>[2x]M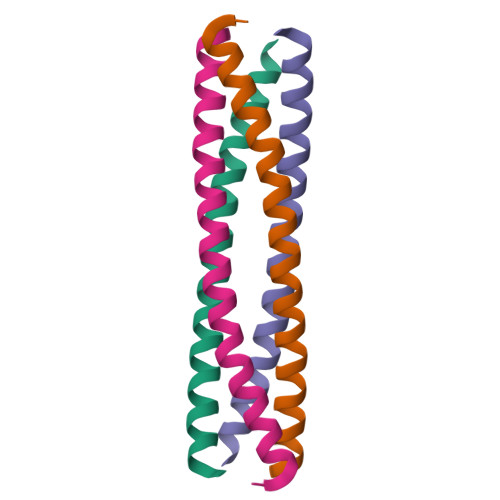TKQEKTALNMARFIRSQTLTLLEKLNELADICESLHDHADELYRSCLARFGDDGENL>[2x]MTKAVPDKFQGFAVSDPKNWNRPKLASYERKQINPHDVVLKNEVCGLCYSDIHTLSAGWQPLQRDNLVVGHEIIGEVIAVGDEVTEFKVGDRVGIGAASSSCRSCQRCDSDNEQYCKQGAATYNSKDVRSNNYVTQGGYSSHSIADEKFVFAIPEDLPSSYGAPLMCAGITVFSPLIRNLGLDARGKNVGIIGIGGLGHLALQFANAMGANVTAFSRSSSKKEQAMKLGAHDFVATGEDKTWY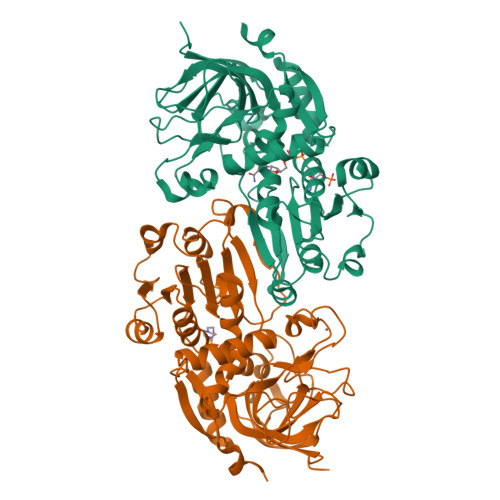KNYDDHFDFILNCASGIDGLNLSEYLSTLKVDKKFVSVGLPPSEDKFEVSPFTFLQQGASFGSSLLGSKTEVKEMLNLAAKHNVRPMIEEVPISEENCAKALDRCHAGDVRYRFVFTDFDKAFKA NMR and X-ray crystallography reveal that Leishmania has a unique type of N-terminally-extended cap-binding protein (eIF4E4) that binds via a PAM2 motif to PABP1. Exceptionally, therefore, by binding tightly to two protein ligands and to the mRNA 5′ cap4 structure, the trypanosomatid N-terminally extended form of eIF4E acts as the core molecular scaffold for the mRNA-cap-binding complex. Thus, in Leishmania, the chain of interactions 5′cap4-eIF4E4–PABP1-poly(A) bridges the mRNA 5′ and 3′ ends. Finally, the eIF4E4 N-terminal extension is an intrinsically disordered region that transitions to a partly folded form upon binding to PABP1, whereby this interaction is not modulated by poly(A) binding to PABP1.

In further work, we were able to solve the crystal structures of PABP1(J) and of PABP1(J) co-crystallized with a synthetic eIF4E4 PAM2 peptide, both to a resolution of ∼2 Å. The structure of the complex reveals how the eIF4E4 peptide binds across the three α-helical segments of the 70-residue PABC domain of PABP1 in a similar fashion to other PABC-interacting proteins. The peptide includes the PAM2 motif (MNPNATEFMP) of eIF4E4, which follows the same pattern of PAM2 motifs found in other proteins, including Paip1 and eRF3 [Φ-(P/V)-A—F-P (34)]. The eIF4E4 peptide in the crystal structure assumes an extended conformation, whereby the PAM2 motif wraps around the core KITGMFLE motif of the PABC domain of PABP1. The phenylalanine (F525) in the PABC core motif of Leishmania PABP1 (KITGMFLE) represents a variation on the MLLE motif generally found in other poly(A)-binding proteins; this residue is located on α-helix 3 and forms part of a hydrophobic pocket that interacts with M140 in the eIF4E4 sequence. A144 in eIF4E4 fits into the hydrophobic pocket formed partially by the PABP1 G523 that also sits on α-helix 3. The carbonyl oxygens of both P142 and A144 interact with the Nϵ atom of K520 at the N-terminal end of α-helix 3. It is also noteworthy that the crystal structure indicates that M148 is angled away from (and does not interact with) P519, although our NMR data reveal that the M148 backbone amide undergoes a significant change in its environment upon binding to PABP1.

>MHHHHHHHHHHHHLPPITPQELESMSPQEQRAALGDRLFLKVYEIAPELAPKITGMFLEMKPKEAYELLNDQKRLEERVTEALCVLKAHQTA[2x];>HHMNPNATEFMPGR[2x]>[8x]MTVVPENFVPGLDGVVAFTTEIAEPDKDGGALRYRGVDIEDLVSQRVTFGDVWALLVDGNFGSGLPPAEPFPLPIHSGDVRVDVQAGLAMLAPIWGYAPLLDIDDATARQQLARASVMALSYVAQSARGIYQPAVPQRIIDECSTVTARFMTMWQGEPDPRHIEAIDAYWVSAAEHGMNASTFTARVIASTGADVAAALSGAIGAMSGPLHG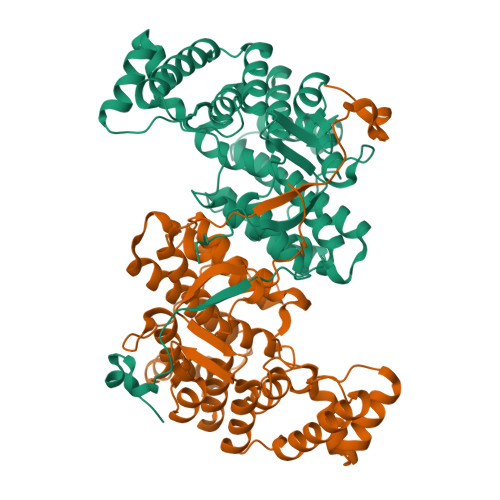GAPARVLPMLDEVERAGDARSVVKGILDRGEKLMGFGHRVYRAEDPRARVLRAAAERLGAPRYEVAVAVEQAALSELRERRPDRAIETNVEFWAAVVLDFARVPANMMPAMFTCGRTAGWCAHILEQKRLGKLVRPSAIYVGPGPRSPESVDGWERVLTTA> MGDVSYIVDSLGLPPFSYQMSLLSFTEKGPQELLQLLSDVFSTISPKHQKVDVAKEVPDQTADRLIGFLKIIKYRPNVQDPLLFRQLVAAGDRETLYQILRWVVPQAQLLE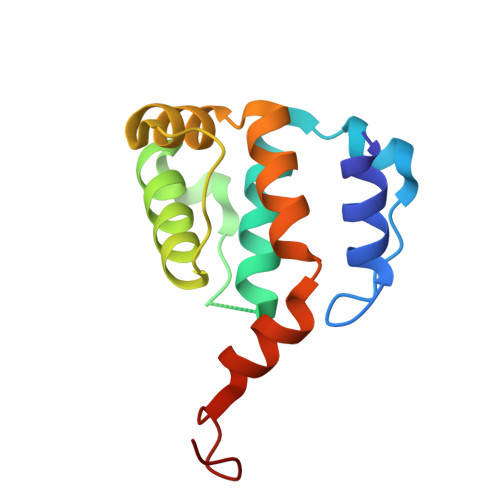KRAFVGYYLSFPD>MSIRTVGIVGAGTMGNGIAQACAVVGLNVVMVDISDAAVQK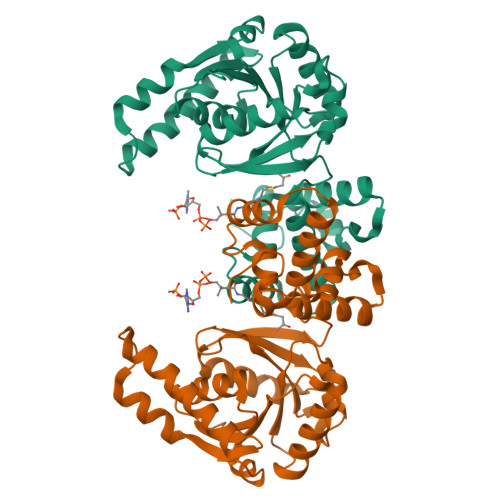GVATVASSLDRLIKKEKLTEADKASALARIKGSTSYDDLKATDIVIEAATENYDLKVKILKQIDGIVGENVIIASNTSSISITKLAAVTSRADRFIGMHFFNPVPVMALVELIRGLQTSDTTHAAVEALSKQLGKYPITVKNSPGFVVNRILCPMINEAFCVLGEGLASPEEIDEGMKLGCNHPIGPLALADMIGLDTMLAVMEVLYTEFADPKYRPAMLMREMVAAGYLGRKTGRGVYVYSK[9x]> MNIFRLTGDLSHLAAIIILLLKIWKSRSCAGISGKSQLLFALVFTTRYLDLFTSFISLYNTSMKLIYIACSYATVYLIYMKFKATYDGNHDTFRVEFLIVPVGGLSFLVNHDFSPLEILWTFSIYLESVAILPQLFMISKTGEAETITTHYLFFLGLYRALYLVNWIWRYYFEGFFDLIAVVAGVVQTVLYCDFFYLYVTKVLKGKKLSLPA;> EHDEL

In the archetypal KDEL-retrieval system, a seven-transmembrane receptor captures escaped ER luminal proteins carrying a C-terminal KDEL or variant tetrapeptide sequence in the mildly acidic pH of the Golgi. Signal binding to a luminal cavity in the receptor triggers a conformational change in its cytoplasmic face, exposing a lysine motif recognised by the COP I coat complex. Hence, the KDEL receptor cycles between the ER and Golgi capturing escaped ER proteins in a dynamic retrieval process. Our previous work has shown the KDEL receptor has a transporter-like architecture and undergoes pH-dependent closure around cognate retrieval signals.

We then determined structures for chicken KDELR2 bound to HDEL and RDEL signals. These structures with TAEHDEL and TAERDEL peptides have resolutions of 2.24 and 2.31 Å, respectively. In both instances the overall structure of the receptor is similar to our previous complex with the TAEKDEL peptide, with a root mean square deviation (R.M.S.D.) of 0.223 and 0.153 Å over 200 Cα atoms for the HDEL and RDEL structures, respectively. Both HDEL and RDEL peptides are bound in a vertical orientation with respect to the membrane, with the side chains clearly resolved in the electron density map. For the histidine side chain at the −4 position of HDEL, the imidazole group is predicted to form a π-π stacking interaction with W120. The higher affinity for HDEL is due to the stronger π-π interaction between the histidine of the −4 position of the retrieval signal and W120 in the receptor. In good agreement with previously reported studies on the mammalian KDEL receptor, we found that HDEL has the highest affinity for the receptor KD 0.24 µM, followed by KDEL KD 1.94 µM and RDEL KD 2.71 µM. To understand the consequences of these changes we examined their positions relative to the bound TAEHDEL signal. This reveals that E117 and S54 sit close to the −4 histidine and −5 glutamate, respectively and D50 is over 5 Å away from any residue in the signal in the final bound state. For the HDEL variant, protonation of both histidine 12 in the receptor and histidine at the −4 position of the retrieval signal favour binding to the receptor in the Golgi.>MGHHHHHHGSTELTPDQQTL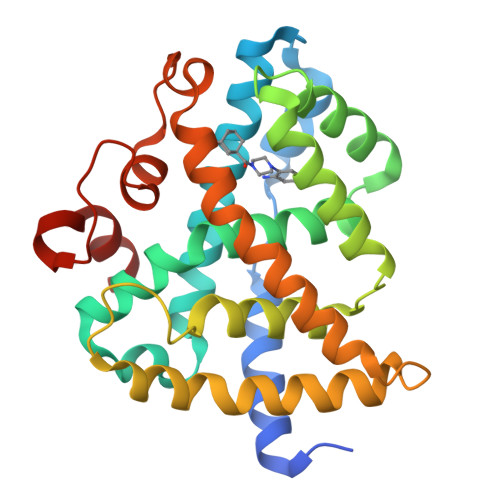LHFIMDSYNKQRMPQEITNKILKEAFSAEENFLILTEMATNHVQVLVEFTKKLPGFQTLDHEDQIALLKGSAVEAMFLRSAEIFNKKLPSGHSDLLEARIRNSGISDEYITPMFSFYKSIGELKMTQEEYALLTAIVILSPDRQYIKDREAVEKLQEPLLDVLQKLCKIHQPENPQHFACLLGRLTELRTFNHHHAEMLMSWRVNDHKFTPLLCEIWDVGSGSGSGSGDHQLLRYLLDKD[2x]>[3x]MNGKFADGPYSGILDSVLDAIGNTPMVRMKRLAKVYGLECDLLAKCEFMSAGGSVKDRIGKAMVEKAEREGRLKAGDTLIEPTSGNTGIGLALAAAVRGYRMIVTMPAKMSAEKSNIMKCLGAEIVRTPTEAA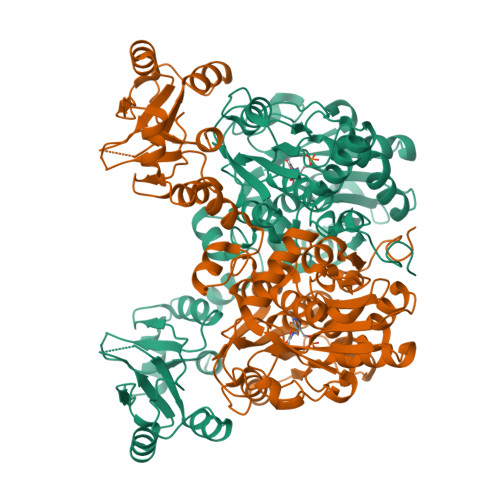WNDENSHMGVAAKLQRELENAHILDQYNNTANPMVHYDVTAEEIITQCDGDIDMVVIGAGTGGTITGIGRKIKERCPKCKVVGVDPKGSILAVPDSLNDEKRLQSYEVEGIGYDFVPGVLDRKVVDEWVKVGDAESFTTARAIIRNEGLFVGGSSGANVWGALQAARQLKKGQKCVVLLPDSSRNYMSKFISDEWMAEHGFAPEDGAKVKEREKQFGGARIRDLLSETGATSDVPFVTARLSVEDVIKMMHETKVKEVIVTEDSEADGKTKLVGVLSEDHIAHSLQSGRCAMQSPVKDIAFKKLAKALPSAYLRDVAKALDFSPYVCVMDEKPRECPHFLGVITRIDLLHWLATKQK> ELTPDQQTLLHFIMDSYNKQRMPQEITNKILKEEFSAEENFLILTEMATNHVQVLVEFTKKLPGFQTLDHEDQIALLKGSAVEAMFLRSAEIFNKKLPSGHSDLLEERIRNSGISDEYITPMFSFYKSIGELKMTQEEYALLTAIVILSPDRQYIKDREAVEKLQEPLLDVLQKLCKIHQPENPQHFACLLGRLTELRTFNH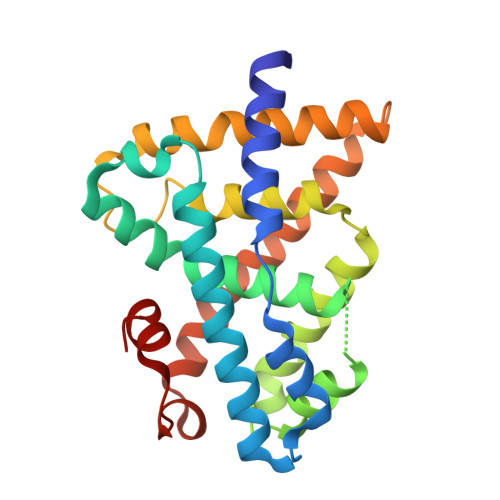HHAEMLMSWRVNDHKFTPLLCEIWDVQ>AISDADLKYLRRCVDLAREALDDGDEPFGSVLVDHTGTTLFEDRNRVKDGDATAHPEFAIARWAARHLTPDRRARATVYTSGEHCPMCAAAHAWVGLGRIVYATSSAQLGGWLTEWGAQAPPVATLPINTVA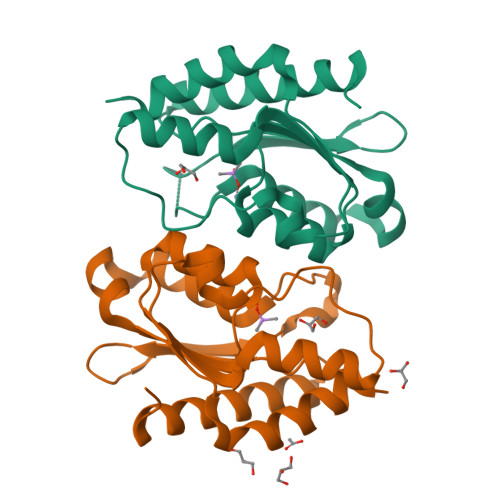PGVVVDGPAEELAETMHNLYRAKFGR[2x]> MGSSHHHHHHSQDPIEGRAQVINTFDGVADYLQTYHKLPDNYITKSEAQALGWVASKGNLCDVAPGKSIGGDIFSNREGKLPGKSGRTWREADINYTCGFRNS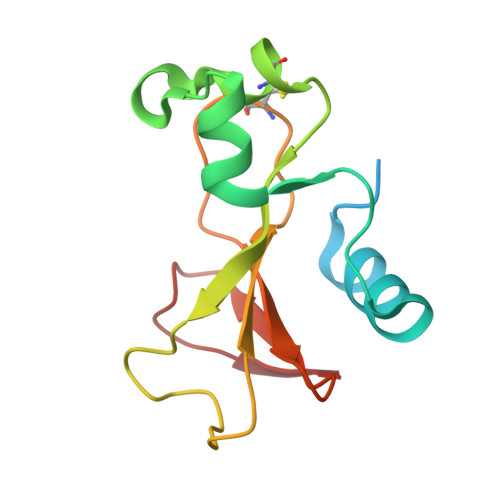DRILYSSDWLIYKTTDHYQTFTKIR> VPMDCSRYPNTTSEEGKVMILCNKALNPVCGTDGVTYDNECVLCAHNLEQGTSVGKKHD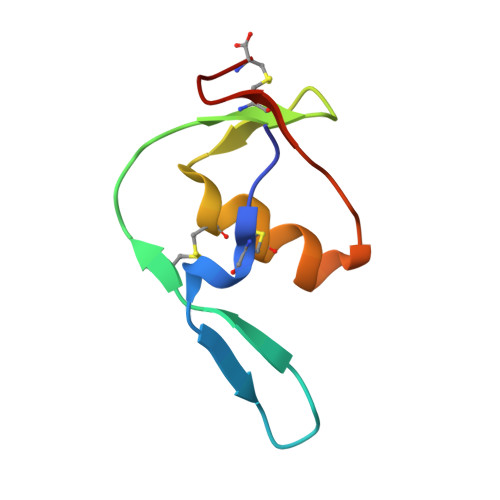GEC TatD is a conserved protein widely expressed in different species, including bacteria, fungi, plants and animals. Here we provide lines of evidence showing that TatD is a 3′–5′ exonuclease that processes single-stranded DNA in DNA repair. TatD represents the first example of a TIM-barrel exonuclease that hydrolyzes the phosphodiester bond at the 3′ end of a nucleic acid chain. TatD has a TIM-barrel fold and it trims DNA from 3′-to-5′ ends in the hydrogen peroxide-induced DNA repair, including double-strand break repair and nucleotide excision repair in E. coli.

To characterize the biochemical properties and examine the structural basis of TatD in DNA degradation, the full-length E. coli TatD with a C-terminal His-tag was expressed and purified by chromatographic methods using a Ni-NTA affinity column followed by a Q-Sepharose anion exchange column. The gel filtration profile showed that TatD formed a stable monomer with a molecular weight of ∼30 kDa at pH 7.2. TatD has a TIM-barrel fold, forming a barrel made of eight β-strands surrounding by nine α-helices. The electrostatic surface potential of TatD revealed an acidic pocket on the top loop region of the β barrel with a patch of basic surface next to the pocket. This acidic pocket is likely the metal-ion binding site and the basic surface on the side with several basic residues, including R98, R129 and R219, is likely involved in DNA binding. Since the E. coli TatD does not bear these two histidine residues, very likely it belongs to the Group I TatD that are activated by Mg2+ but not by Zn2+. Therefore, based on the structure comparison of the active site of TatD, E. coli TatD resembles more closely to the group I TatD and likely binds two or three Mg2+ ions in the active site for DNA hydrolysis. In summary, we suggest that the conserved acidic residues E91, E201 and D203 are responsible for binding of metal ions, and H62 for playing a critical catalytic role in the active site of E. coli TatD in DNA hydrolysis.

> MFDIGVNLTSSQFAKDRDDVVACAFDAGVNGLLITGTNLRESQQAQKLARQYSSCWSTAGVHPHDSSQWQAATEEAIIELAAQPEVVAIGECGLDFNRNFSTPEEQERAFVAQLRIAADLNMPVFMHCRDAHERFMTLLEPWLDKLPGAVLHCFTGTREEMQACVAHGIYIGITGWVCDERRGLELRELLPLIPAEKLLIETDAPYLLPRDLTPKPSSRRNEPAHLPHILQRIAHWRGEDAAWLAATTDANVKTLFGIAFLE> MELAEKDKGRDFTLRNARMDDIDQIIKINRLTLPENYPYYFFVEHLKEYGLAFFVAIVDNSVVGYIMPRIEWGFSNIKQLPSLVRKGHVVSIAVLEEYRRKGIATTLLEASMKSMKNDYNAEEIYLEVRVSNYPAIALYEKLNFKKVKVLKGYYADGEDAYLMARPLHHHHHH;> SSGTPT

Nα-acetyltransferase (Nat) performs this modification and transfers an acetyl group from acetyl-coenzyme A (acetyl-CoA) to an α-amino group from the first residue of the protein substrate. A BLAST search identified Ard1 from Crenarchaeal Sulfolobus solfataricus (SsArd1) as a homolog of the Ard1 subunit of yeast NatA and Naa10p subunit of human NatA. However, no Sulfolobus homolog of the auxiliary subunit of NatA was found, so SsArd1 alone may be responsible for the protein acetylation. SsArd1 has a mixed α/β-fold with 7 β-sheet surrounded by 4 α-helices and contains 4 conserved motifs, a feature unique to the GCN5-related N-acetyltransferase (GNAT) family.

The crystal structure of the SsArd1-CoA binary complex was determined at 2.13 Å resolution and the SsArd1–CoA/peptide ternary complex at 1.84 Å. CoA-bound and CoA/peptide-bound SsArd1 structures were almost identical and could be superimposed, with root mean square deviation (RMSD) 0.12 Å for all Cα atoms. In the crystal structure of the SsArd1–CoA/peptide complex, we identified a clear electron-dense Fo–Fc map corresponding to the first 2 residues of the 6-mer Alba peptide. The Alba peptide fragment is located in the pocket formed between the α1-α2 loop, β6-β7 loop, and β4 and β5. The first 2 residues of Alba bound to SsArd1 via a number of van der Waals interactions and hydrogen bonds. The main-chain of Glu127 and side-chain of Tyr154 interacted with the main-chain of the first residue Ser by a hydrogen bond. In addition, the main-chain carbonyl of the second Ser formed a hydrogen bond to the side-chain of Tyr37. Structural alignment of ternary complexes of SsArd1 and hNaa50p revealed that residues of substrate binding for hNaa50p, Val29, His112, Tyr138 and Tyr139 were located in almost the same orientation and overlapped with the residues Glu35, Glu127, Tyr153 and Tyr154 for SsArd1. A comparison of Val29 of hNaa50p and Glu35 of SsArd1 in these ternary complexes showed that the side-chain of Glu35 from SsArd1 is too close and features steric clashes against the side-chain of the first Met residue of the substrate for hNaa50p. Residue Glu35 of SsArd1 may play a critical role for substrate specificity in Nα-acetylation.>[2x]MVPISPIETVPVKLKPGMDGPKVKQWPLTEEKIKALVE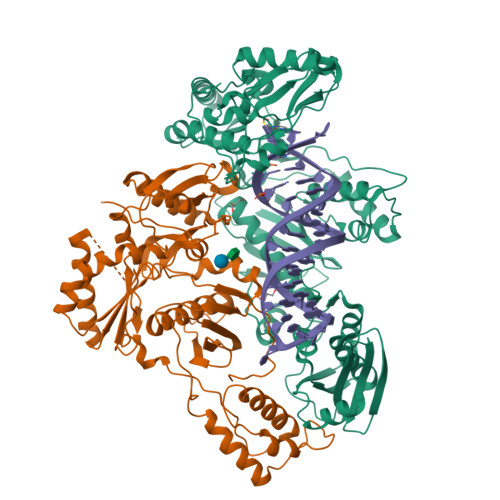ICTEMEKEGKISKIGPENPYNTPVFAIKKKDSTKWRKLVDFRELNKRTQDFWEVQLGIPHPAGLKQKKSVTVLDVGDAFYSVPLDKDFRKYTAFTIPSINNETPGIRYQYNVLPMGWKGSPAIMQSSMTKILEPFRKQNPDIVIYQYVDDLYVGSDLEIGQHRTKIEELRQHLLRWGFTTPDKKHQKEPPFLWMGYELHPDKWTVQPIVLPEKDSWTVNDIQKLVGKLNWASQIYAGIKVRQLSKLLRGTKALTEVVPLTEEAELELAENREILKEPVHGVYYDPSKDLIAEIQKQGQGQWTYQIYQEPFKNLKTGKYARMKGAHTNDVKQLTEAVQKIATESIVIWGKTPKFKLPIQKETWEAWWTEYWQATWIPEWEFVNTPPLVKLWYQLEKEPIIGAETFYVDGAANRETKLGKAGYVTDRGRQKVVPLTDTTNQKTELQAIHLALQDSGLEVNIVTDSQYALGIIQAQPDKSESELVSQIIEQLIKKEKVYLAWVPAHKGIGGNEQVDKLVSAG;>[2x]MAHHHHHHALEVLFQGPISPIETVPVKLKPGMDGPKVKQWPLTEEKIKALVEICTEMEKEGKISKIGPENPYNTPVFAIKKKDSTKWRKLVDFRELNKRTQDFWEVQLGIPHPAGLKQKKSVTVLDVGDAYFSVPLDKDFRKYTAFTIPSINNETPGIRYQYNVLPQGWKGSPAIFQSSMTKILEPFRKQNPDIVIYQYMDDLYVGSDLEIGQHRTKIEELRQHLLRWGFTTPDKKHQKEPPFLWMGYELHPDKWTVQPIVLPEKDSWTVNDIQKLVGKLNWASQIYAGIKVRQLSKLLRGTKALTEVVPLTEEAELELAENREILKEPVHGVYYDPSKDLIAEIQKQGQGQWTYQIYQEPFKNLKTGKYARMKGAHTNDVKQLTEAVQKIATESIVIWGKTPKFKLPIQKETWEAWWTEYWQATWIPEWEFVNTPPLVKLWYQ> LSNISMSSSEIIDVLCENLNDGIWALRVLYAEGAMNKEKLWDYINQYHKDYQIENEKDYEGKKILPSRYA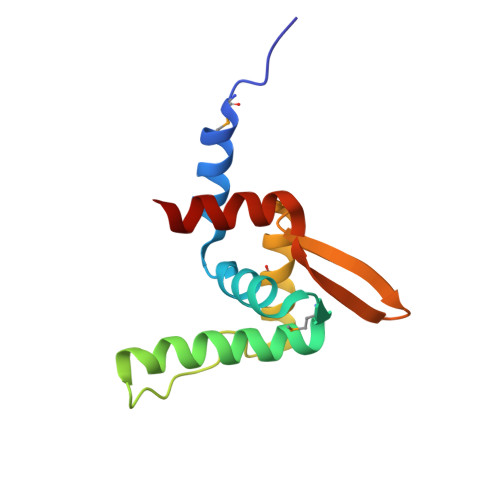LDIMTARLEGAGLISFKAIGRVRIYDVTDLGNVLIKELEKR>[2x]MSLHASAIESIETIIVDLPTIRPHKLAMHTMQNQTLVLIRLRCADGIEGLGESTTIGGLAYGNESPDSIKTNIDRFVAPLLIGQDASN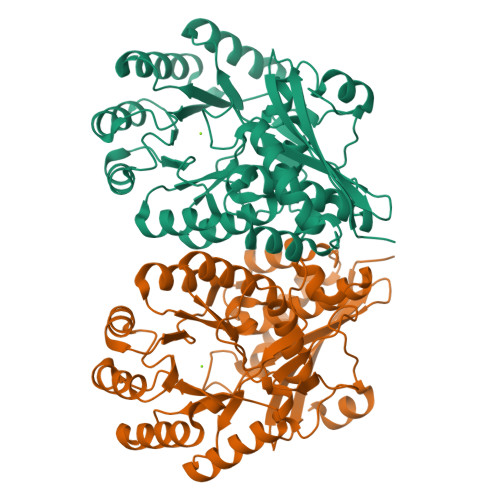INAAMLRLEQSIRGNTFAKSGIESALLDAQGKRLGLPVSELLGGRVRDALPVAWTLASGDTAKDIAEAQKMLDLRRHRIFKLKIGAGEVDRDLAHVIAIKKALGDSASVRVDVNQAWDEAVALRACRILGGNGIDLIEQPISRNNRAGMVRLNASSPAPIMADESIECVEDAFNLAREGAASVFALKIAKNGGPRATLRTAAIAEAAGIGLYGGTMLEGGIGTLASAHAFLTLNKLSWDTELFGPLLLTEDILAEPPVYRDFHLHVSKAPGLGLSLDEERLAFFRREGHHHHHH> STPNDPRFDDQWHYYEQAGGLNLPTAWDTATGSGVVVAVLDTGYRPHADLNANILPGYDMISNLSVANDGGGRDSDARDPGDAVAANECGTNGAQNSSWHGTHVAGTVAA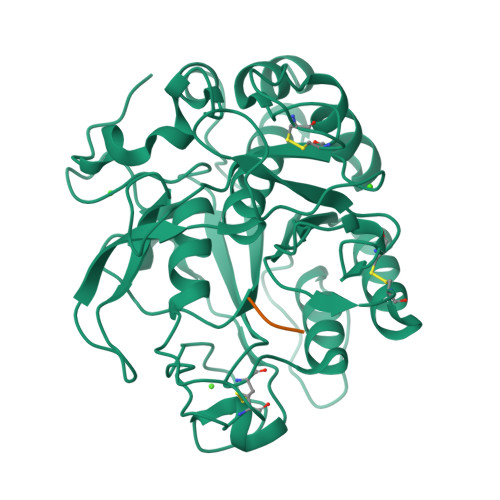VTNNGEGVAGVAYNAKVVPVRVLGKCGGLTSDIADGIIWASGGSVSGIPANSNPADVINMSLGGSGSCSSTTQNAINTARSNGTVVVIAAGNDNDNSANYNPGNCNGVVNVASVGRNGGRAYYSNYGSNIDVAAPGGAQSFANDSEGVLSTYNSGSSTPSSDSYGYSQGTSMAAPHVAGVAALIKQAKPDATPDEIESILKSTTRSFPATCTSCGTGIVDAAAAVAAASKGHHHHHH[(2~{R},3~{S},4~{S},5~{S},6~{S})-3,4,5,6-tetrakis(oxidanyl)oxan-2-yl]methyl hexadecanoate | C22 H42 O7 | 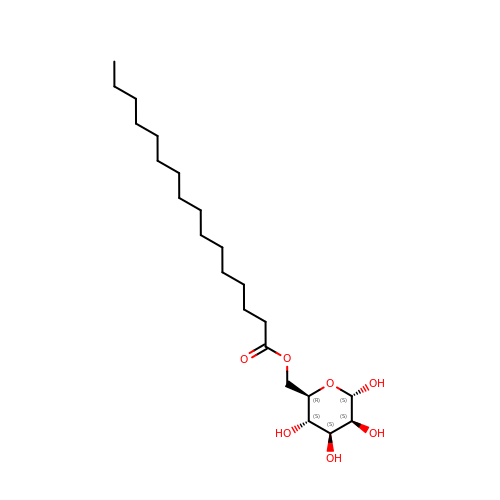JTWNPFJEQQORKD-ICGSVKGVSA-N1,5-dimethyl-3-naphthalen-1-yl-6-(2-oxidanyl-6-oxidanylidene-cyclohexen-1-yl)carbonyl-quinazoline-2,4-dione | C27 H22 N2 O5 | 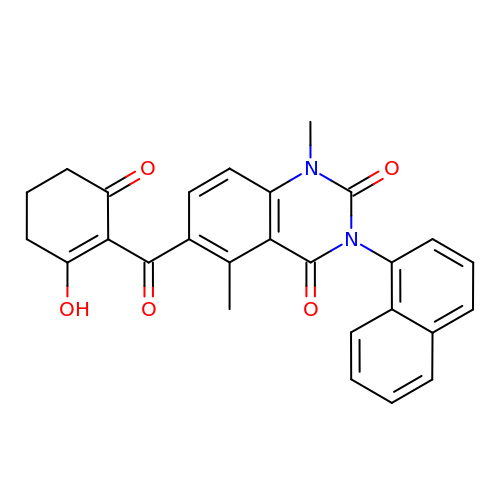PDXPJCZVXMZTSY-UHFFFAOYSA-N>SNAASARSVRVLVDMDGVLADFEAGLLRGFRRRFPEEPHVPLEQRRGFLAREQYRALRPDLADKVASVYEAPGFFLDLEPIPGALDAVREMNDLPDTQVFICTSPLLKYHHCVGEKYRWVEQHLGPQFVERIILTRDKTVVLGDLLIDDKDTVRGQEETPSWEHILFTCCHNRHLVLPPTRRRLLSWSDNWREILDSKRGAAQ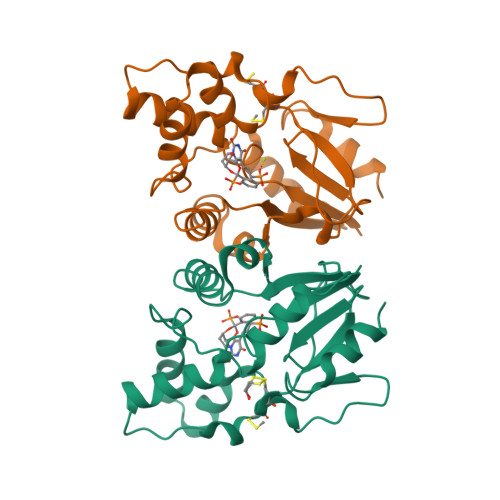RE[2x]>[2x]MKKRLAYAIIQFLHDQLRHGGL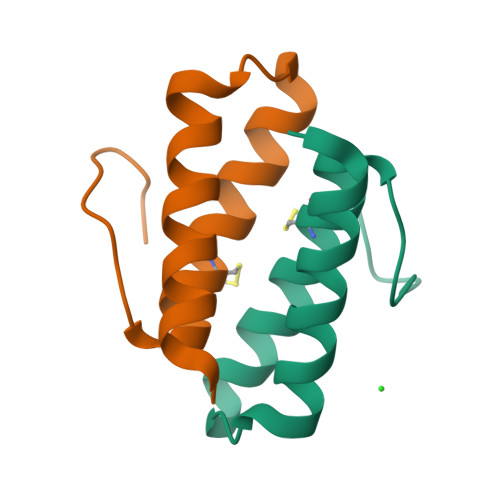SSDAQESLEVAIQCLETAFGVTVEDSDLAL>[2x]MSDRKPVRGRHQAR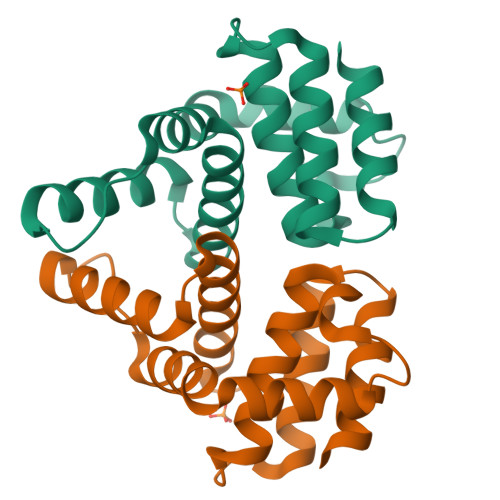KRAVALLFEAEVRGISAAEVVDTRAALAEAKPDIARLHPYTAAVARGVSEHAAHIDDLITAHLRGWTLDRLPAVDRAILRVSVWELLHAADVPEPVVVDEAVQLAKELSTDDSPGFVNGVLGQVMLVTPQLRAAAQAVRGGA>MHHHHHHGSDDDDKRPEAKSAQPADGWKGERPRSEEDNELNLPNLAAAYSSILSSLGENPQRQGLLKTPWRAASAMQFFTKGYQETISDVLNDAIFDEDHDEMVIVKDIDMFSMCEHHLVPFVGKVHIGYLPNKQVLGLSKLARIVEIYSRRLQVQERLTKQIAVAITEALRPAGVGVVV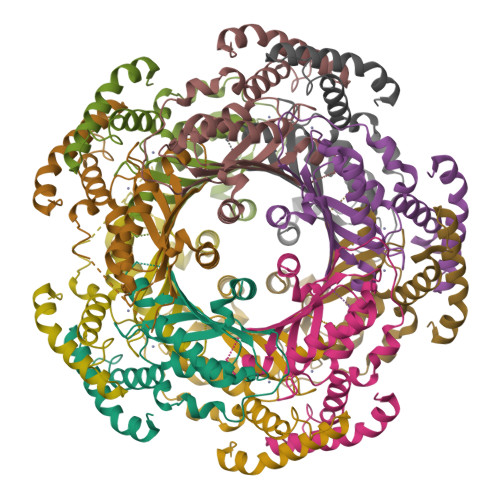EATHMCMVMRGVQKMNSKTVTSTMLGVFREDPKTREEFLTLIRS[5x]> MNGVLLRHQQPGGLGRAPRKPMPRGASRLVAKEPLSVRLPKADFSFLKYLAWPLLLAVLGYGAYRGAEYILPYADRPIAKVSVEGDLSYISQRAVQQRISPYLAASFFTIDLAGMRGQLEQMPWIAHAEVRRVWPDQVVIRLDEQLPIARWGDEALLNNQGQAFTPKELANYEHLPRLHGPQRAQQQVMQQYQLLSQLLRPLGFSIARLEMSDRGGWALTTAQGVEIQIGRDHVVDKIRRFVSIYDKALKDQISNIARIDLRYPNGLAVAWREPV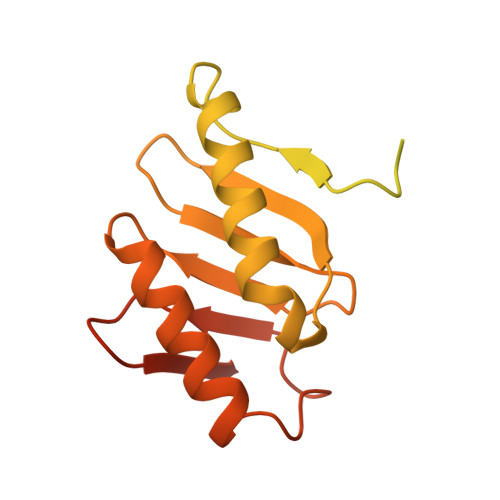TPATVATASAVQ>QQASTLPDLAEQFAPPDVAPPLLIKLVEAIEKKGLECSTLYRTQSSSNPAELRQLLDCDTASLDLEMFDVHVLADAFKRYLLDLPNPVIPVAVSSELISLAPEVQSSKEYIQLLKKLIRSPSIPHQYWLTLQYLLKHFFKLSQTSSKNLLNARVLSELFSPLLFRFPAASSENTEHLIKIIEILISTEWNERQ[2x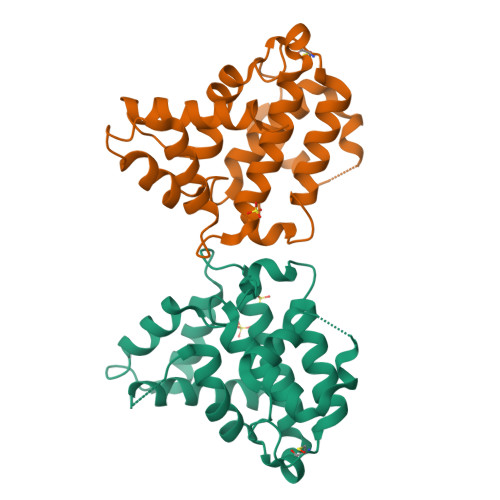]> MWPPRLLSCIFTIILIVAVIAPTSDSTTVRRRLRKPSKSVSVTSSVSRSTDQVISASVNRPKIRGRPSVASRKSSAALDNSVGTDDH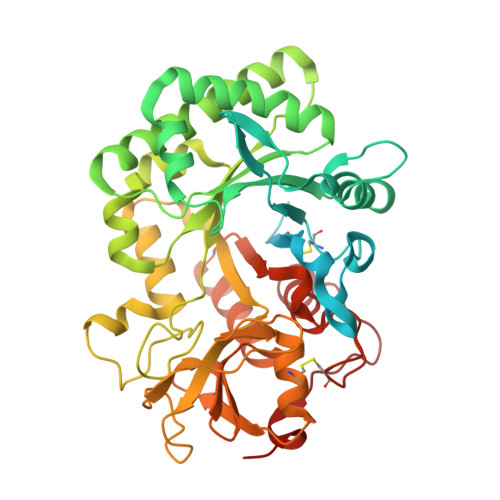KDKDGYKIVCYYTNWSQYRTKIGKFMPEDIQPELCTHIIFAFGWLKKGKLSSFESNDETKDGKTGLYDRINALKKANPKLKTLLAIGGWSFGTQKFKEMSATRYARQTFIYSAIPYLRDRNFDGLDIDWLYPKGGDDKKNYVLLLKELREAFEAEAQEVKKPRLLLTAAVPVGPDNIKSGYDVPAVASYLDFINLMAYDFHGKWERETGHNAPLYAPSSDSEWRKQLSVDHAAHLWVKLGAPKEKLIIGMPTYGRTFTLSNPNNFKVNSPASGGGKAGEYTKESGFLAYYEVCEILRNGGAYVWDDEMKVPYAIHGDQWVGFDDEKSIRNKMRWIKDNSFGGAMVWTVDMDDFSGGVCGGNVKYPLIGAMREELRGISRGKDAKDVDWASVAASV>MNHKVHHHHHHIEGRHMTELKSKFVKVYSVLKKELLHDSAFGLTDDSRNWVERIMDYNVPGGKLNRGLSVVDSYKLLRELTNSKYKSELSDDEIFLASVLGWSVEWIQACALVLDDIMDHSHTRRGHPCWFRLPKVGMIAINDGLILRNHVPRILRTHFQTEHYYLQLVDLFHEVECQTIAGQMLDLI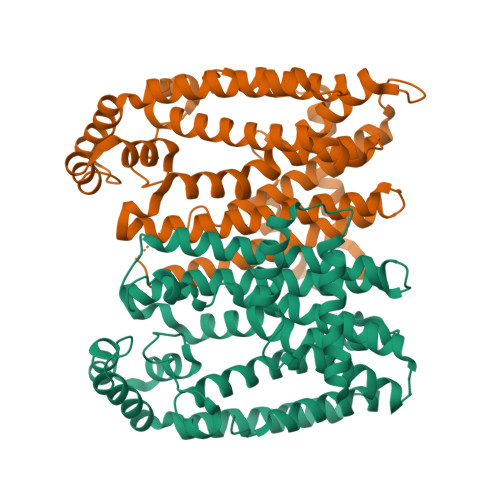TTLAGEINLSSYSLPVYQQITLSKTSYYSFYLPVACALVMLGENLESHDDMKDILLEMGTYFQVQDDYLDCFGDPEVIGKIGTDIEDNKCTWLVVQALEHCNEEQKKLLYDNYGRKDPKQVAKVKELYKTLNLEDLFTQYENKTCKKLTKSIEALPNVAVQAVLKSFLAKIHKRLK[2x]> SNAMTNSSEKQWERIQQLEKEHVEVYRELLITLDRLYLIRKHNHAVILSHTQQRLLEIRHQLQINLEKTALLIRLLEKPDNTNVLFTKLQNLLEE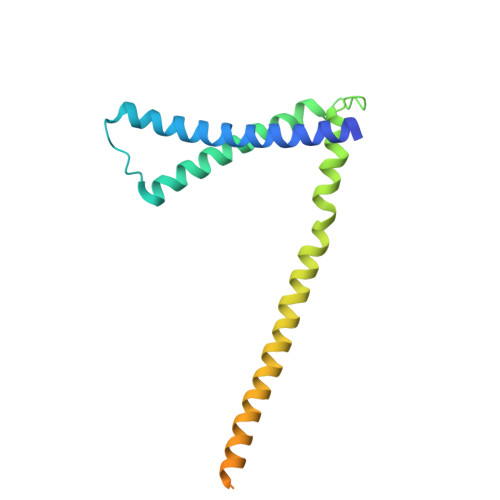SNSLDYELLQSLGAQSSLHKQLIESRAERDELMSKLIELSSKFPKPTIPPDDSDTAGKQVEVEKENETIQELMIALQIHSGYTNISYTI> DWWPLAFEAL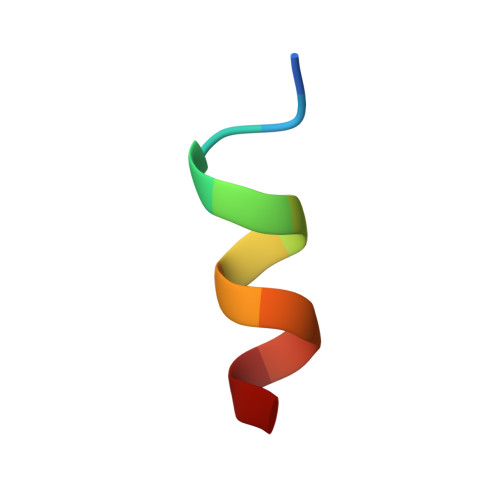LR SUCCINAMIDE-COA | C25 H41 N8 O19 P3 | 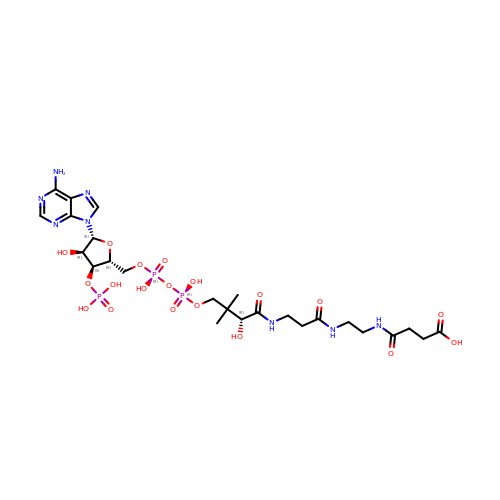WZEXTLJNSXEEHK-ITIYDSSPSA-N> SLDQVENQAIPDPPCTCKYKKEIEDLGENSVPRFIETRNCQKTQQPTCR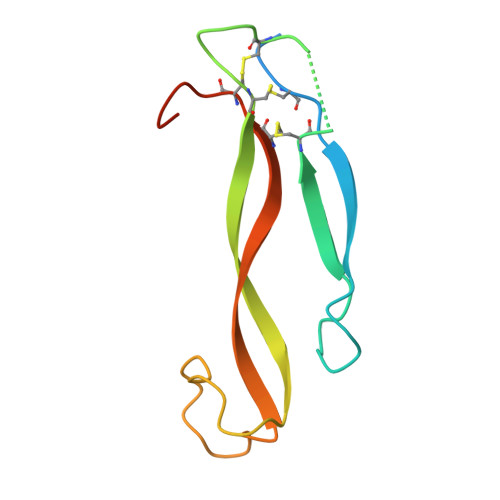PPYICKESLYSITILKRRETKSQESLEIPNELKYRWVAESHPVSVACLCTRDYQLRYNNN BlaC is a class A serine β‐lactamase found in Mycobacterium tuberculosis (Wang et al., 2006). The enzymes in this class utilize an active site serine (Ser70) to perform a nucleophilic attack on β‐lactam rings, forming a covalent acyl‐enzyme intermediate that is subsequently hydrolyzed (Fisher & Mobashery, 2009; Strynadka et al., 1992). BlaC can efficiently hydrolyze penicillin antibiotics but has low activity against later‐generation oxyimino‐cephalosporins, such as ceftazidime, due to their bulky C7β aminothiazole‐oxyimino side chain (Sun et al., 2023; Wang et al., 2006). We analyzed the structural changes in mutants of the β‐lactamase BlaC from Mycobacterium tuberculosis obtained via directed evolution for increased ceftazidime hydrolysis activity.

In a screen for BlaC mutants with improved ceftazidime resistance in an Escherichia coli expression system at three temperatures (23, 30, and 37°C), the BlaC variant P167S/D240G (PD) was found at 30°C, exhibiting a 16‐fold increased resistance for ceftazidime as compared to the wild‐type (WT). Grown at 23 and 37°C, the resistance of this PD variant was eightfold greater than that of WT. The crystal structures of BlaC variants PD, PDDS, and PDDSH were solved at 1.3, 1.6, and 1.4 Å resolution, respectively. For BlaC PD, the Ω‐loop exhibits a large conformational change compared to WT, resulting in a significant expansion of the active site cavity (yellow), in line with the changes observed for BlaC P167S (green), which were attributed to the cis‐to‐trans change in the peptide bond between residues 166 and 167 (Sun et al., 2023). The parent variant for evolution, PD, showed a melting temperature (T m) of 52.8°C, a decrease of 9.2°C compared to WT BlaC (62°C) (van Alen et al., 2023). The yield of soluble protein of variant PD was reduced relative to that of WT BlaC. In the P167S and PD variants, peak doubling is observed for many amides, indicating that a large part of the protein populates two states. Stability loss is also clearly observed when selecting for enhanced ceftazidime activity in BlaC, as indicated by a decrease in the melting temperature of more than 9°C for the PD mutant and more than 11°C for the PDTT mutant. For one branch of the directed evolution experiment, we managed to obtain crystal structures of the successive mutants, PD, PDDS, and PDDSH, showing the opening and increasing disorder of the Ω‐loop in an otherwise defined protein structure, suggesting minor structural changes.

> ADLADRFAELERRYDARLGVYVPATGTTAAIEYRADERFAFCSTFKAPLVAAVLHQNPLTHLDKLITYTSDDIRSISPVAQQHVQTGMTIGQLCDAAIRYSDGTAANLLLADLGGPGGGTAAFTGYLRSLGDTVSRLDAEESELNRDPPGDERDTTTPHAIALVLQQLVLGNALPPDKRALLTDWMARNTTGAKRIRAGFPADWKVIDKTGTGGYGRANDIAVVWSPTGVPYVVAVMSDRAGGGYDAEPREALLAEAATCVAGVLA>SMLDVGNAEVKLEEENRSLKADLQKLK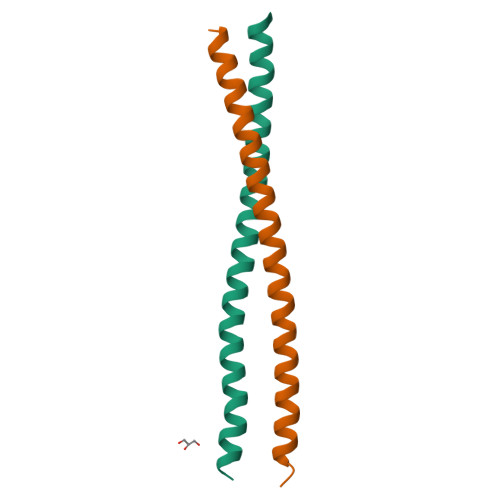DELASTKQKLEKAENQVLAMRKQSEGLTKEYDRLLEEHAKL[4x]>RQNWEEADSMKSSVESLQNRVTELESVDKSAGQVARNTGLLESQLSRHDQMLSVHDIRLADMDLRFQVLETASYNGVLIWKIRDYKRRKQEAVMGKTLSLYSQPFYTGYFGYKMCARVYLNGDGMGKGTHLSLFFVIMRGEYDALLPWPFKQKVTLMLMDQGSSRRHLGDAFKPDPNSSSFKK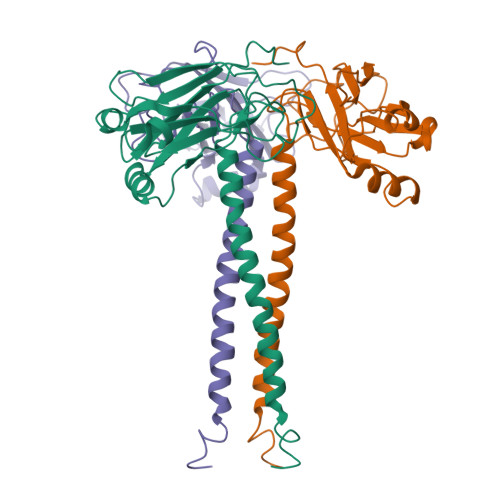PTGEMNIASGCPVFVAQTVLENGTYIKDDTIFIKVIVDTSDLPDP[2x]> AFVVTDNCIKCKY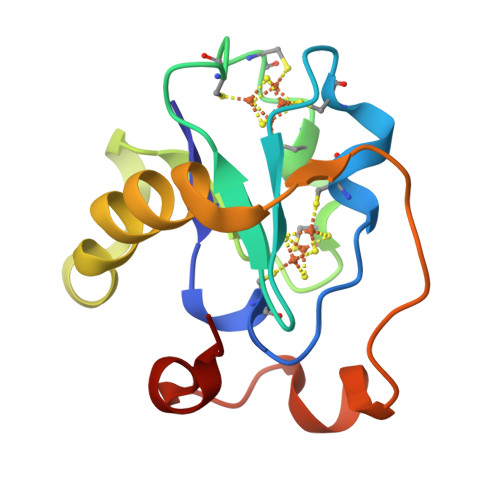TDCVEVCPVNCFYEGPNFLVIHPDECIDCALCEPECPAQAIFSEDEVPEDMQEFIQLNAELAEVWPNITEKKDPLPDAEDWDGVKGKLQHLER> SMNPIEDELVFRVGSRGREKGEFTNLQGVSAASSGRIVVADSNNQCIQVFSNEGQFKFRFGVRGRSPGQLQRPTGVAVDTNGDIIVADYDNRWVSIFSPEGKFKTKIGAGRLMGPKGVAVDRNGHIIVVDNKSCCVFTFQPNGKLVGRFGGRGATDRHFAGPHFVAVNNKNEIVVTDFHNHSVK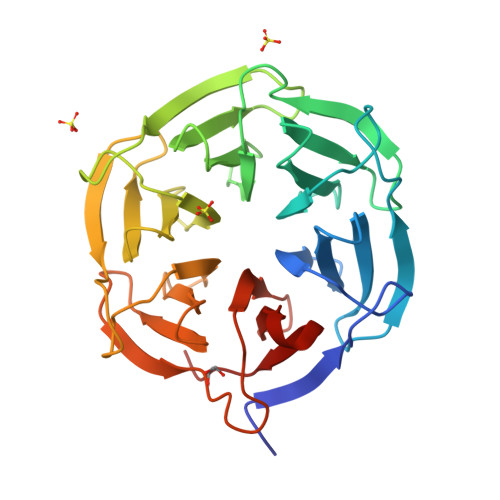VYSADGEFLFKFGSHGEGNGQFNAPTGVAVDSNGNIIVADWGNSRIQVFDSSGSFLSYINTSAEPLYGPQGLALTSDGHVVVADAGNHCFKAYRYLQ> MDPSSRDSQRNLLVIALLFVSFMIWQAWEQDKNPQPQAQQTTQTTTTAAGSAADQGVPASGQGKLISVKTDVLDLTINTRGGDVEQALLPAYPKELNSTQPFQLLETSPQFIYQAQSGLTGRDGPDNPANGPRPLYNVEKDAYVLAEGQNELQVPMTYTDAAGNTFTKTFVLKRGDYAVNVNYNVQNAGEKPLEISSFGQLKQSITLPPHLDTGSSNFALHTFRGAAYSTPDAAYAAYAFDTIADNENLNISSKGGWVAMLQQYFATAWIPHNDGTNNFYTANLGNGIAAIGYKSQPVLVQPGQTGAMNSTLWVGPEIQDKMAAVAPHLDLTVDYGWLWFISQPLFKLLKWIHSFVGNWGFSIIIITFIVRGIMYPLTKAQYTSMAKMRMLQPKIQAMRERLGDD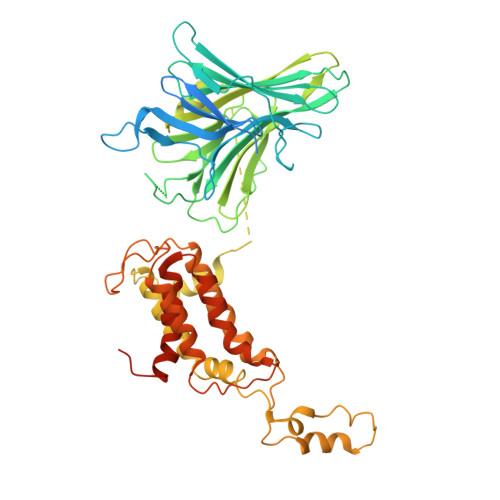KQRISQEMMALYKAEKVNPLGGCFPLLIQMPIFLALYYMLMGSVELRQAPFALWIHDLSAQDPYYILPILMGVTMFFIQKMSPTTVTDPMQQKIMTFMPVIFTVFFLWFPSGLVLYYIVSNLVTIIQQQLIYRGLEKRGLHSREKKKSHHHHHH> MKCLVTGGNVKVLGKAVHSLSRIGDELYLEPLEDGLSLRTVNSSRSAYACFLFAPLFFQQYQAATPGQDLLRCKILMKSFLSVFRSLAMLEKTVEKCCISLNGRSSRLVVQLHCKFGVRKTHNLSFQDCESLQAVFDPASCPHMLRAPARVLGEAVLPFSPALAEVTLGIGRGRRVILRSYHEEEADSTAKAMVTEMCLGEEDFQQLQAQEGVAITFCLKEFRGLLSFAESANLNLSIHFDAPGRPAIFTIKDSLLDGHFVLATLS;> HMKFRAKIVDGACLNHFTRISNMIAKLAKTCTLRISPDKLNFILCDKLANGGVSMWCELEQENFFNEFQMEGVSAENN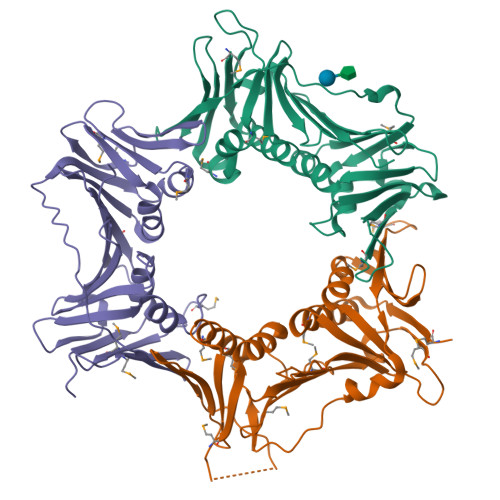EIYLELTSENLSRALKTAQNARALKIKLTNKHFPCLTVSVELLSMSSSSRIVTHDIPIKVIPRKLWKDLQEPVVPDPDVSIYLPVLKTMKSVVEKMKNISNHLVIEANLDGELNLKIETELVCVTTHFKDLGNPPLASESTHEDRNVEHMAEVHIDIRKLLQFLAGQQVNPTKALCNIVNNKMVHFDLLHEDVSLQYFIPALS;> DQYSLVASLDNVRNLSTILKAIHFREHATCFATKNGIKVTVENAKCVQANAFIQAGIFQEFKVQEESVTFRINLTVLLDCLSIFGSSPMPGTLTALRMCYQGYGYPLMLFLEEGGVVTVCKINTQEPEETLDFDFCSTNVINKIILQSEGLREAFSELDMTSEVLQITMSPDKPYFRLSTFGNAGSSHLDYPKDSDLMEAFHCNQTQVNRYKISLLKPSTKALVLSCKVSIRTDNRGFLSLQYMIRNEDGQICFVEYYCCPDE>GSGDSGSPGIATPLVLGENLCSINGWVPTYRGEGTTGKIPDEQMLTRQNFVSCSDKECRRFFVSMGYGTTTNFADLIVSEQMNVYSVKLGDPPTPDKLKFEAVGWSASSCHDGFQWTVLSVAGDGFVSILYGGIITDTIHPTNGGPLRTQASSCICNDGTCYTIIADGTTYTASSHRLYRLVNGTSAGWKALDTTGFNFEFPTCYYTSGKVKCTGTNLWNDAKRPFLEFDQSFTYTFKEPCLGFLGDTPRGIDTTNYCDKTTTEGEGGIQGFMIEGSNSWIGRIINPGSKKGFEIYKFLGTLFSVQTVGNRNYQLLSNSTIGRSGLYQPAYESRDCQELCFWIEIAATTKAGLSSND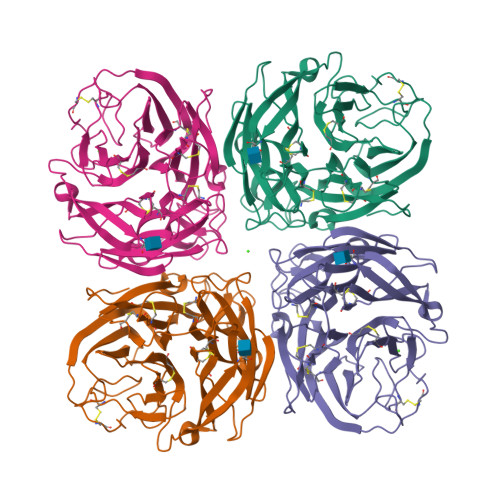LITFCGTGGSMPDVNWG[4x]>[4x]GKSAVIFVERATPATLTELKDALSNSILSVRDPWSIDFRTYRCSIKNLPADVSKLMYSITFHHHGRQTVLIKDNSAMVTTAAAADIPPALVFNGSSTGVPESIDTILSSKLSNIWMQRQLIKGDAGETLILDGLTVRLVNLFSSTGFKGLLIELQADEAGEFETKIAGIEGHLAEIRAKEYKTSSDSLGPDTSNEICDLAYQYVRALEL;>VQQLSLFGSIGDDGYDLLISTLTTISGNPPLLYNSLCTVWKPNPSYDVENVNSRNQLVEPNRIKLSKEVPFSYLIDETMMDKPLNFRILKSFTNDKIPLNYAMTRNILHNTVPQVTNFNSTNEDQNNSKH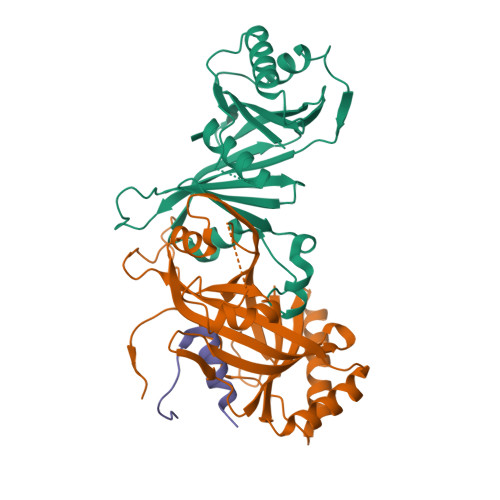TEDTVNESRNSDDIIDVDMDASPAPSNESCSPWSLQISDIPAAGNNRSVSMQTIAETIILSSAGKNSSVSSLMNGLGYVFEFQYLTIGVKFFMKHGLILELQKIWQIEEAGNSQITSGGFLLKAYINVSRGTDIDRINYTETVLMNLKKELQGYIELSVPDRQSMDSRVAHGNILI[4x];>SKPSKPFNVDDVLKFTFTGEKHHHHHH[4x]> MLSRKGIIPEEYVLTRLAEDPTEPRYRTRERRARFVSKKGNCNVAHKNIREQGRFLQDVFTTLVDLKWPHTLLIFTMSFLCSWLLFAMVWWLIAFAHGDLAPGEGTNVPCVTSIHSFSSAFLFSIEVQVTIGFGGRMVTEECPLAILILIVQNIVGLMINAIMLGCIFMKTAQAHRRAETLIFSKHAVITPRHGRLCFMLRVGDLRKSMIISATIHMQVVRKTTSPEGEVVPLHQVDIPMENGVGGNSIFLVAPLIIYHVIDSNSPLYDLAPSDLHHHQDLEIIVILEGVVETTGITTQARTSYLADEILWGQRFVPIVAEEDGRYSVDYSKFGNTVKVPTPLCTARQLDEDRSLLDALTLASSRGPLRKRSVAVA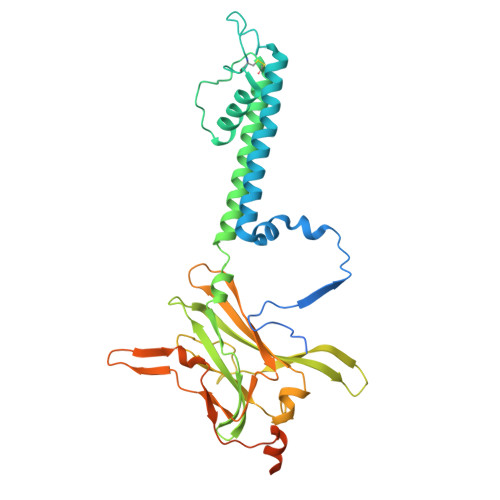KAKPKFSISPDSLS>GSSGSSGEPVQDTPPTELHFGEKWFHKKVESRTSAEKLLQ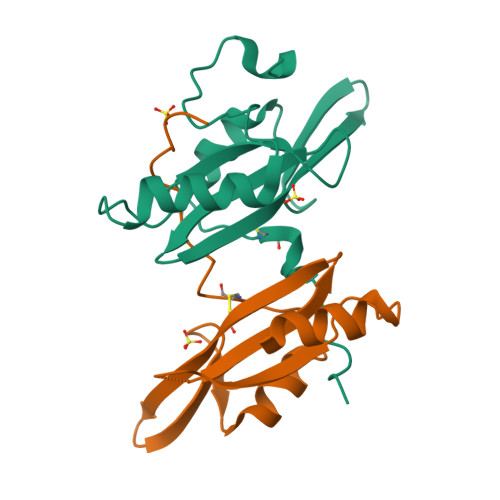EYCAETGAKDGTFLVRESETFPNDYTLSFWRSGRVQHCRIRSTMENGVMKYYLTDNLTFNSIYALIQHYREAHLRCAEFELRLTDPVPNPNPSGPSSG[2x]>MTQTAAKSLKFPKDFLWGAATAAYQIEGAANEDGRGPSIWDTFSHTPGKVHNGDNGDVACDHYHRYKEDVELMKELGLNAYRFSISWPRILPEGEGKVNQKGLDFYNNLIDELLENGIEPFVTLYHWDLPQALQDKGGWENRETVDAFAEYARVCFERFGDRVKYWITFNEPNVFAVLGYLSGVHPPGMKDLKKAFRAAHNLLLAHARAVKAYREISQNGQIGITLNLSPVYPASDNEEEDKAAAERADQFNNWFLDPIFKGKYEHMLERLGEQIAANGGELPEITDEMEILSASLDFIGLNYYTSNLVRANPNSGSSSVKPPDLPRTDMGWEIYPEGLYDLLKRIHEKYNLPIYITENGMAVDDEVEDGAVHDTNRIDYLKEHLEAVHKAIEEGVNVRGYFVWSLMDNFEWANGYSKRFGLIYVDYKTQKRTPKKSAYWYREVIKSNGLELEHHHHHH[2x]

Family 1 glycosidases (GH1) commonly function as β-glucosidases and β-galactosidases, although other activities are also found in the family. GH1 enzymes are present in the three domains of life and have been traced back to LUCA23. We focus on a putative ancestor of modern bacterial and eukaryotic enzymes and find a number of unusual properties that clearly differentiate the ancestor from the properties of its modern descendants. Unexpectedly, the ancestral glycosidase binds heme tightly at a well-defined site in the structure with concomitant allosteric increase in enzyme activity.

Furthermore, there is a large region missing in the electronic density map of the ancestral protein from X-ray crystallography, while the rest of the model agrees with a homology model based on modern glycosidase structures. At the achieved resolution of 2.5 Å, it should be possible to trace the course of a polypeptide chain in space, provided that such course is well defined. Therefore, the missing regions very likely correspond to regions of high flexibility. In addition, flexibility is also suggested by the B-factor values in regions that are present in the ancestral structure. That is, the missing regions in the X-ray structure match the high-flexibility regions in the molecular dynamics simulations and include the proteolysis cleavage sites determined by mass spectrometry. Overall, regions encompassing two alpha helices and several loops appear to be highly flexible or even unstructured in the ancestral glycosidase. The barrel core, however, remains structured and shows comparatively low conformational flexibility, which may explain the high thermal stability of the protein (see Discussion). The ancestral glycosidase is highly susceptible to proteolysis and degradation is already apparent after only a few minutes incubation at a low concentration of thermolysin (0.01 mg/mL). Overall, the comparatively low activity of the ancestral protein is likely linked to its conformational flexibility.>LLEKRPEDVVIVAANRSAIGKGFKGAFKDVNTDYLLYNFLNEFIGRFPEPLRADLNLIEEVACGNVLNVGAGATEHRAACLASGIPYSTPFVALNRQCSSGLTAVNDIANKIKVGQIDIGLALGVESMTNNYKNVNPLGMISSEELQKNREAKKCLIPMGITNENVAANFKISRKDQDEFAANSYQKAYKAKNEGLFEDEILPIKLPDGSICQSDEGPRPNVTAESLSSIRPAFIKDRGTTTAGNASQVSDGVAGVLLARRSVANQLNLPVLGRYIDFQTVGVPPEIMGVGPAYAIPKV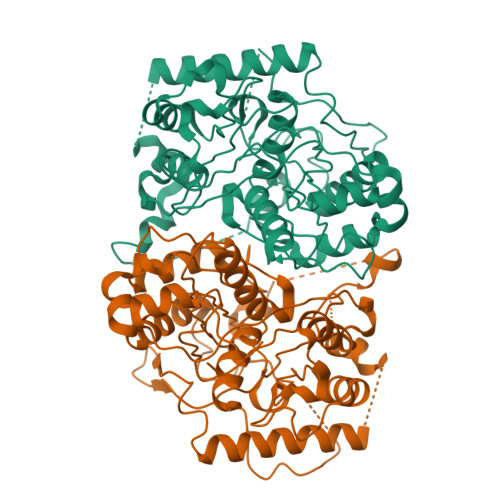LEATGLQVQDIDIFEINEAFAAQALYCIHKLGIDLNKVNPRGGAIALGHPLGCTGARQVATILRELKKDQIGVVSMCIGTGMGAAAIFIKE[2x]2-methyl-~{N}-[(1~{S})-1-thieno[3,2-b]pyridin-6-ylethyl]pyridin-3-amine 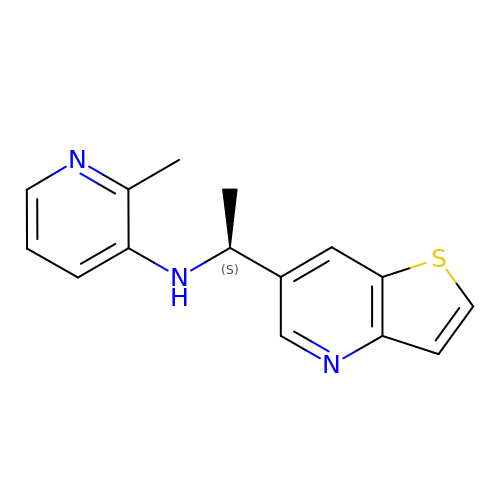| C15 H15 N3 S | BHXCHKMTMFQWLX-JTQLQIEISA-N> MLKQVEIFTDGSCLGNPGPGGYGAI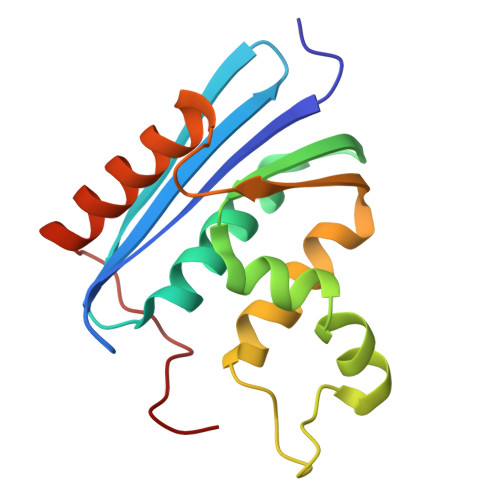LRYRGREKTFSAGYTRTTNNRMELMAAIVALEALKEACEVILSTDSQYVRQGITQWIHNWKKRGWKTADKKPVKNVDLWQRLDAALGQHQIKWEWVKGHAGHPENERCDELARAAAMNPTLEDTGYQVEV> MSFQITPTRDLKVITDELQTLSSYIFHTNIVDDLNSLLTWMSPNDAKSNHQLRPPSLRIKNIIKVLFPNNATTSPYSMINTSQANNSIVNEGNTNKELQLQLFSTLKEFYIFQVRYHFFLHFNNINYLKDIQRWENYYEFPLRYVPIFDVNVNDWALELNSLRHYLLNRNIKFKNNLRTRLDKLIMDDDFDLADNLIQWLKSANGSLSSTELIVNALYSKINKFCEDNMSRVWNKRFMIMETFNKFINQYWSQFSKLVGCPEDDHELTTTVFNCFESNFLRIRTNEIFDICVLAYPDSKVTLLELRKIMKDFKDYTNIVTTFLSDFKKYILNPSVTTVDALLRYVKTIKAFLVLDPTGRCLHSITTFVKPYFQERKHLVNVLLYAMLDLPEEELKEKINFNVDMKALLSLVDTLHDSDINQDTNITKRDKNKKSPFLWNLKVKGKRELNKDLPIRHAMLYEHILNYYIAWVPEPNDMIPGNIKSSYIKTNLFEVLLDLFESREFFISEFRNLLTDRLFTLKFYTLDEKWTRCLKLIREKIVKFTETSHSNYITNGILGLLETTAPAADADQSNLNSIDVMLWDIKCSEELCRKMHEVAGLDPIIFPKFISLLYWKYNCDTQ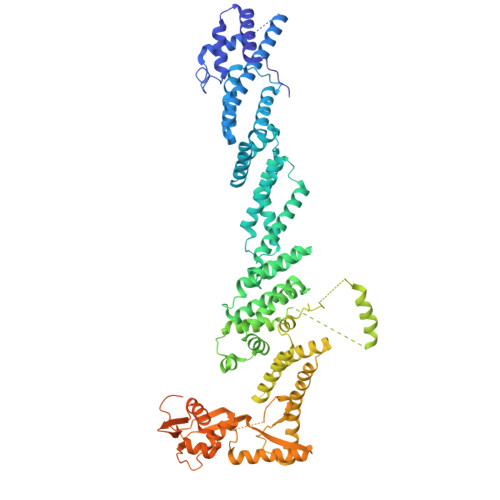GSNDLAFHLPIDLERELQKYSDIYSQLKPGRKLQLCKDKGKVEIQLAFKDGRKLVLDVSLEQCSVINQFDSPNDEPICLSLEQLSESLNIAPPRLTHLLDFWIQKGVLLKENGTYSVIEHSEMDFDQAQKTAPMEIENSNYELHNDSEIERKYELTLQRSLPFIEGMLTNLGAMKLHKIHSFLKITVPKDWGYNRITLQQLEGYLNTLADEGRLKYIANGSYEIVKNGHKNS>GEDGYIADGDNCTYICTFNNYCHALCTDKK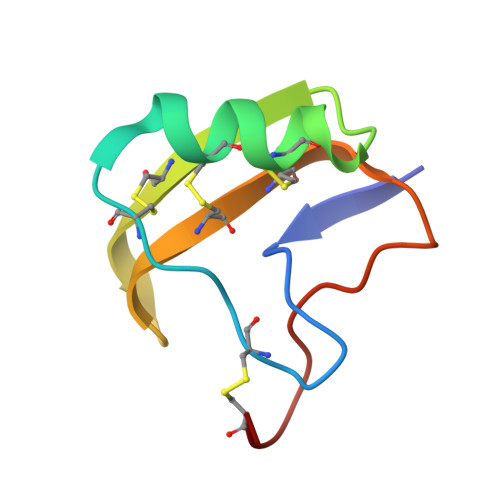GDSGACDWWVPYGVVCWCEDLPTPVPIRGSGKCR[2x]>CGVGFIAAIDGKPRRSVVEKGIEALKAVWHRGAVDADGKTGDGAGIHVAVPQKFFKDHVKVIGHRAPDNKLAVGQVFLPRISLDAQEACRCIVETEILAFGYYIYGWRQVPINVDIIGEKANATRPEIEQIIVGNNKGVSDEQFELDLYIIRRRIEKAVKGEQINDFYICSLSARSIIYKGMFLAEQLTTFYPDLLDERFESDFAIYHQRYSTNTFPTWPLAQPFRMLAHNGEINTVKGNVNWMKAHETRMEHPAFGTHMQDLKPVIGVGLSDSGSLDTVFEVMVRAGRTAPMVKMMLVPQALTSSQTTPDNHKALIQYCNSVMEPWDGPAALAMTDGRWVVGGMDRNGLRPMRYTITTDGLIIGGSETGMVKIDETQVIEKGRLGPGEMIAVDLQSGKLYRDRELKDHLATLKPWDKWVQNTTHLDELVKTASLKGEPSDMDKAELRRRQQAFGLTMEDMELILHPMVEDGKEAIGSMGDDSPIAVLSDKYRGLHHFFRQNFSQVTNPPIDSLRERRVMSLKTRLGNLGNILDEDETQTRLLQLESPVLTTAEFRAMRDYMGDTAAEIDATFPVDGGPEALRDALRRIRQETEDAVRGGATHVILTDEAMGPARAAIPAILATGAVHTHLIRSNLRTFTSLNVRTAEGLDTHYFAVLIGVGATTVNAYLAQEAIAERHRRGLFGSMPLEKGMANYKKAIDDGLLKIMSKMGISVISSYRGGGNFEAIGLSRALVAEHFPAMVSRISGIGLNGIQKKVLEQHATAYNEEVVALPVGGFYRFRKSGDRHGWEGGVIHTLQQAVTNDSYTTFKKYSEQVNKRPPMQLRDLLELRSTKAPVPVDEVESITAIRKRFITPGMSMGALSPEAHGTLNVAMNRIGAKSDSGEGGEDPARFRPDKNGDNWNSAIKQVASGRFGVTAEYLNQCRELEIKVAQGAKPGEGGQLPGFKVTEMIARLRHSTPGVMLISPPPHHDIYSIEDLAQLIYDLKQINPDAKVTVKLVSRSGIGTIAAGVAKANADIILISGNSGGTGASPQTSIKFAGLPWEMGLSEVHQVLTLNRLRHRVRLRTDGGLKTGRDIVIAAMLGAEEFGIGTASLIAMGCIMVRQCHSNTCPVGVCVQDDKLRQKFVGTPEKVVNLFTFLAEEVREILAGLGFRSLNEVIGRTDLLHQVSRGAEHLDDLDLNPRLAQVDPGENARYCTLQGRNEVPDTLDARIVADARPLFEEGEKMQLAYNARNTQRAIGTRLSSMVTRKFGMFGLQPGHITIRLRGTAG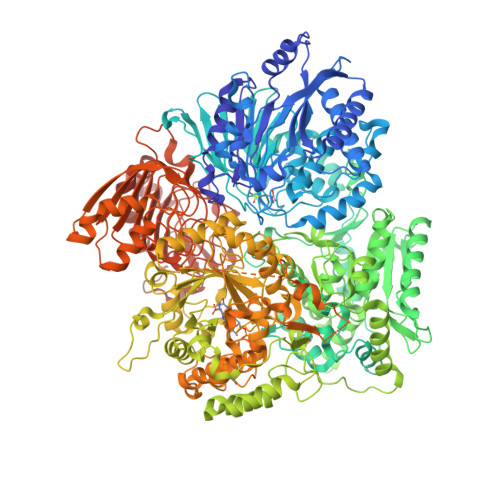QSLGAFAVQGIKLEVMGDANDYVGKGLSGGTIVVRPTTSSPLETNKNTIIGNTVLYGATAGKLFAAGQAGERFAVRNSGATVVVEGCGSNGCEYMTGGTAVILGRVGDNFAAGMTGGMAYVYDLDDSLPLYINDESVIFQRIEVGHYESQLKHLIEEHVTETQSRFAAEILNDWAREVTKFWQVVPKEMLNRLEVPVHLPKAISAE[2x]4-(3-methoxy-5-methylphenoxy)-2-(4-methoxyphenyl)-6-methylpyridine | C21 H21 N 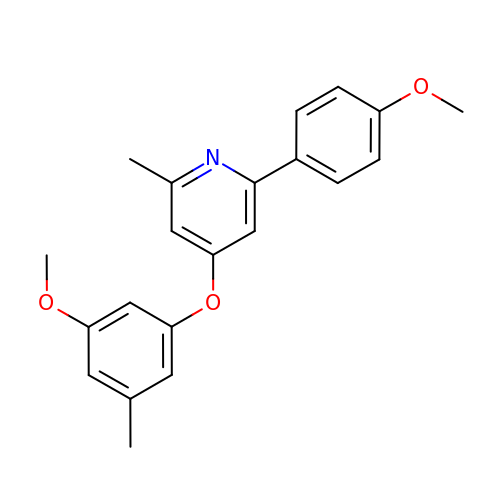O3 | WAAJEIGWGSZNPQ-UHFFFAOYSA-N> GXGTACA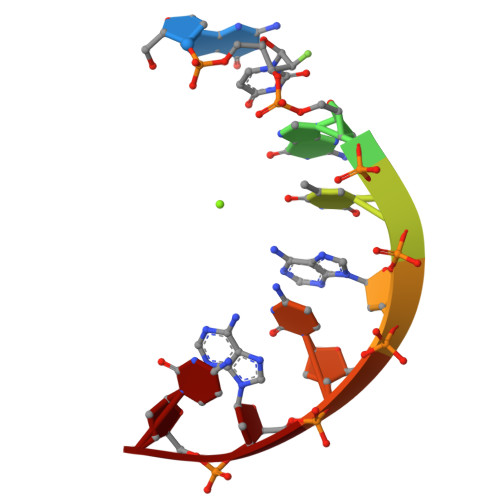C>FNLDTEELTAFRVDSAGFGDSVVQYANSWVVVGAPQKITAANQTGGLYQCGYSTGACEPIGLQVPPEAVNMSLGLSLASTTSPSQLLACGPTVHHECGRNMYLTGLCFLLGPTQLTQRLPVSRQECPRQEQDIVFLIDGSGSISSRNFATMMNFVRAVISQFQRPSTQFSLMQFSNKFQTHFTFEEFRRSSNPLSLLASVHQLQGFTYTATAIQNVVHRLFHASYGARRDAAKILIVITDGKKEGDSLDYKDVIPMADAAGIIRYAIGVGLAFQNRNSWKELNDIASKPSQEHIFKVEDFDALKDIQNQLKEKIFAIEGTETTSSSSFELEMAQEGFSAVFTPDGPVLGAVGSFTWSGGAFLYPPNMSPTFINMSQENVDMRDSYLGYSTELALWKGVQSLVLGAPRYQHTGKAVIFTQVSRQWRMKAEVTGTQIGSYFGASLCSVDVDSDGSTDLVLIGAPHYYEQTRGGQVSVCPLPRGWRRWWCDAVLYGEQGHPWGRFGAALTVLGDVNGDKLTDVVIGAPGEEENRGAVYLFHGVLGPSISPSHSQRIAGSQLSSRLQYFGQALSGGQDLTQDGLVDLAVGARGQVLLLRTRPVLWVGVSMQFIPAEIPRSAFECREQVVSEQTLVQSNICLYIDKRSKNLLGSRDLQSSVTLDLALDPGRLSPRATFQETKNRSLSRVRVLGLKAHCENFNLLLPSCVEDSVTPITLRLNFTLVGKPLLAFRNLRPMLAADAQRYFTASLPFEKNCGADHICQDNLGISFSFPGLKSLLVGSNLELNAEVMVWNDGEDSYGTTITFSHPAGLSYRYVAEGQKQGQLRSLHLTCDSAPVGSQGTWSTSCRINHLIFRGGAQITFLATFDVSPKAVLGDRLLLTANVSSENNTPRTSKTTFQLELPVKYAVYTVVSSHEQFTKYLNFSESEEKESHVAMHRYQVNNLGQRDLPVSINFWVPVELNQEAVWMDVEVSHPQNPSLRCSSEKIAPPASDFLAHIQKNPVLDCSIAGCLRFRCDVPSFSVQEELDFTLKGNLSFGWVRQILQKKVSVVSVAEITFDTSVYSQLPGQEAFMRAQTTTVLEKYKVHGCGGLENLYFQ[4x];>[4x]QECTKFKVSSCRECIESGPGCTWCQKLNFTGPGD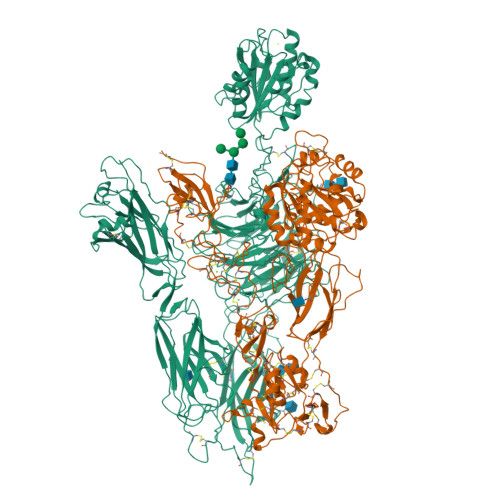PDSIRCDTRPQLLMRGCAADDIMDPTSLAETQEDHNGGQKQLSPQKVTLYLRPGQAAAFNVTFRRAKGYPIDLYYLMDLSYSMLDDLRNVKKLGGDLLRALNEITESGRIGFGSFVDKTVLPFVNTHPDKLRNPCPNKEKECQPPFAFRHVLKLTNNSNQFQTEVGKQLISGNLDAPEGGLDAMMQVAACPEEIGWRNVTRLLVFATDDGFHFAGDGKLGAILTPNDGRCHLEDNLYKRSNEFDYPSVGQLAHKLAENNIQPIFAVTSRMVKTYEKLTEIIPKSAVGELSEDSSNVVQLIKNAYNKLSSRVFLDHNALPDTLKVTYDSFCSNGVTHRNQPRGDCDGVQINVPITFQVKVTATECIQEQSFVIRALGFTDIVTVQVLPQCECRCRDQSRDRSLCHGKGFLECGICRCDTGYIGKNCECQTQGRSSQELEGSCRKDNNSIICSGLGDCVCGQCLCHTSDVPGKLIYGQYCECDTINCERYNGQVCGGPGRGLCFCGKCRCHPGFEGSACQCERTTEGCLNPRRVECSGRGRCRCNVCECHSGYQLPLCQECPGCPSPCGKYISCAECLKFEKGPFGKNCSAACPGLQLSNNPVKGRTCKERDSEGCWVAYTLEQQDGMDRYLIYVDESRECVAGPDGCGENLYFQ> MSPFLYLVLLVLGLHATIHCASPEGKVTACHSSQPNATLYKMSSINADFAFNLYRRFTVETPDKNIFFSPVSISAALVMLSFGACCSTQTEIVETLGFNLTDTPMVEIQHGFQHLICSLNFPKKELELQIGNALFIGKHLKPLAKFLNDVKTLYETEVFSTDFSNISAAKQEINSHVEMQTKGKVVGLIQDLKPNTIMVLVNYIHFKA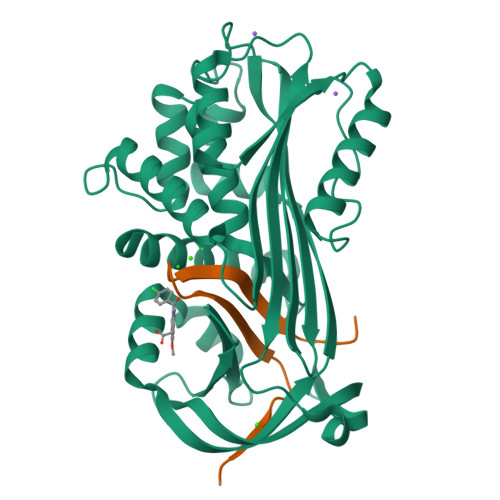QWANPFDPSKTEDSSSFLIDKTTTVQVPMMHQMEQYYHLVDMELNCTVLQMDYSKNALALFVLPKEGQMESVEAAMSSKTLKKWNRLLQKGWVDLFVPKFSISATYDLGATLLKMGIQHAYSENADFSGLTEDNGLKLSNAAHKAVLHIGEKGTEAAGAMFLEAIPR;> HPIIQIDRSFMLLILERSTRSILFLGKVVNPTEA S-{(3R,5R,9R)-1-[(2R,3S,4R,5R)-5-(6-amino-9H-purin-9-yl)-4-hydroxy-3-(phosphonooxy)tetrahydrofuran-2-yl]-3,5,9-trihydroxy-8,8-dimethyl-3,5-dioxido-10,14-dioxo-2,4,6-trioxa-11,15-diaza-3lambda~5~,5lambda~5~-diphosphaheptadecan-17-yl} (5R,10R)-7-hydroxy-10-methyl-2-oxo-1-oxaspiro[4.5]dec-6-ene-6-carbothioate 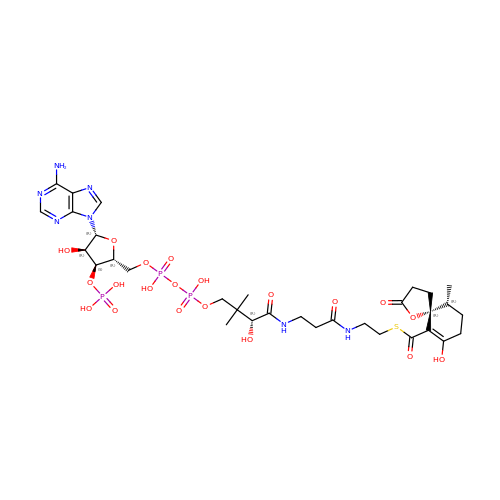(non-preferred name) | C32 H48 N7 O20 P3 S | COMHLEMSBYWTLA-LJKJHTHQSA-N>NLNLPEQSTRFQTIASIHSNNCSFEILNNDPGYIYGDSVDGECRIAVAHRELGNGLERTGDDRFLFIFYALDNNNFIIANRHDGFVLQFLIANGQGVIVSREYQPNIHQEFTIQSINSDTFRLHSRDTNTFATVCWAQFNSWTKIVSRVDNPGAPNANLKHRSLLTDINMPQLPSLTPLQPLPRLTELEDGGLSPAQAPRAIIGRTLIPCLFVNDPVLRLENRIKQSPYYVLEHRQYWHRIWTDIFTAGERREYREVTGINNNAQNDMNKMINITIGADGPNRLRFGNLSTPFRQQIIDNSNTLGSFANTNYGTRTDIVNVFNSEFH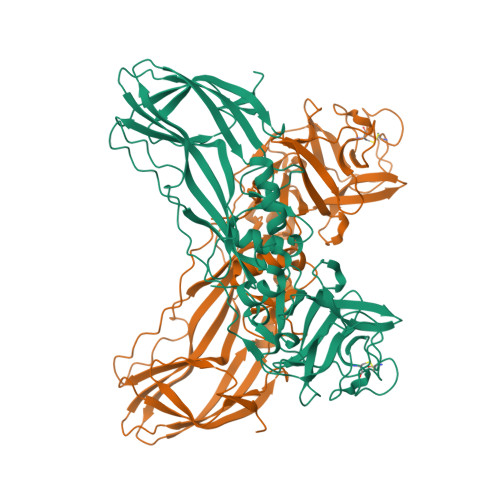QVRYARFVKAYEYRLTRADGSQVGTPWVVLDRKEMDLRTYPHNMAITLENVKIDNADNSYDLSIWKTPLKLKDGKIIIENHENSKPYYN[2x]> KRNYILGLAIGITSVGYGIIDYETRDVIDAGVRLFKEANVENNEGRRSKRGARRLKRRRRHRIQRVKKLLFDYNLLTDHSELSGINPYEARVKGLSQKLSEEEFSAALLHLAKRRGVHNVNEVEEDTGNELSTKEQISRNSKALEEKYVAELQLERLKKDGEVRGSINRFKTSDYVKEAKQLLKVQKAYHQLDQSFIDTYIDLLETRRTYYEGPGEGSPFGWKDIKEWYEMLMGHCTYFPEELRSVKYAYNADLYNALNDLNNLVITRDENEKLEYYEKFQIIENVFKQKKKPTLKQIAKEILVNEEDIKGYRVTSTGKPEFTNLKVYHDIKDITARKEIIENAELLDQIAKILTIYQSSEDIQEELTNLNSELTQEEIEQISNLKGYTGTHNLSLKAINLILDELWHTNDNQIAIFNRLKLVPKKVDLSQQKEIPTTLVDDFILSPVVKRSFIQSIKVINAIIKKYGLPNDIIIELAREKNSKDAQKMINEMQKRNRQTNERIEEIIRTTGKENAKYLIEKIKLHDMQEGKCLYSLEAIPLEDLLNNPFNYEVDHIIPRSVSFDNSFNNKVLVKQEEASKKGNRTPFQYLSSSDSKISYETFKKHILNLAKGKGRISKTKKEYLLEERDINRFSVQKDFINRNLVDTRYATRGLMNLLRSYFRVNNLDVKVKSINGGFTSFLRRKWKFKKERNKGYKHHAEDALIIANADFIFKEWKKLDKAKKVMENQMFEEKQAESMPEIETEQEYKEIFITPHQIKHIKDFKDYKYSHRVDKKPNRELINDTLYSTRKDDKGNTLIVNNLNGLYDKDNDKLKKLINKSPEKLLMYHHDPQTYQKLKLIMEQYGDEKNPLYKYYEETGNYLTKYSKKDNGPVIKKIKYYGNKLNAHLDITDDYPNSRNKVVKLSLKPYRFDVYLDNGVYKFVTVKNLDVIKKENYYEVNSKCYEEAKKLKKISNQAEFIASFYNNDLIKINGELYRVIGVNNDLLNRIEVNMIDITYREYLENMNDKRPPRIIKTIASKTQSIKKYSTDILGNLYEVKSKKHPQIIKKG

Staphylococcus aureus Cas9 (SaCas9) is a widely used genome editing tool. The CRISPR-Cas9 system has been emerging as a simple and powerful genome editing technology and is widely applied to the fields of gene therapy, drug screening, disease model construction, etc.. This system mainly consists of two components: Cas9 endonuclease and single-guide RNA (sgRNA). Additionally, its DNA editing process is roughly as follows: firstly, Cas9 binds to sgRNA to form a ribonucleoprotein (RNP) complex; next, the RNP searches for the protospacer-adjacent motif (PAM) on DNA to locate the target site; meanwhile, ~20 nt guide sequence of the sgRNA tries to pair with the DNA sequences upstream of the PAM; once they are in a form of base pairing, Cas9 endonuclease is activated and then precisely cleaves the target site.

To promote the stable binding of the protein to DNA, we mutated D10 and N580 of the wild-type SaCas9 (wtSaCas9) into alanine and obtained dead SaCas9 (dSaCas9). In this study, we report the first cryo-electron microscopy (cryo-EM) map of the SaCas9-sgRNA-DNA ternary complex. This map reveals that the HNH nuclease domain is tightly bound to the cleavage site of the target DNA strand and closely interacts with the WED and REC domains. Hence, most parts of the SaCas9-sgRNA-DNA complex are distributed in the high-resolution regions of the map, except for the HNH domain, L1/L2 linkers, and a small part of RuvC3 (aa 717–755). The components of the complex model are SaCas9 (aa 2-1053; D10A/N580A), 104 nt sgRNA, 40 nt target DNA strand, and 28 nt non-target DNA strand. In addition, the model shows that the cryo-EM density contacts of the HNH domain with the REC and WED domains are attributed to the hydrogen bonding between the domains: S581 of the HNH domain with E131 of the REC domain, and S595 and R586 of the HNH domain with K811 and D812 of the WED domain, respectively. The model shows that the non-target DNA strand fragment of the PAM upstream stably inserts into the positively charged groove formed by the HNH, L2, RuvC, and PI domains. Significantly, the full-length model also showed the hairpin structure of the stem-loop 2 in the sgRNA and revealed that the stem-loop 2 binds tightly to the positively charged groove formed by the PI and RuvC II domains. In addition, we observed that the double helix in the downstream of PAM is also embedded in the positively charged groove of the PI domain, and the phosphate backbone of dA15 in the target DNA strand binds to K1023 with a hydrogen bond. Site-directed mutagenesis and molecular dynamics (MD) simulations confirmed that the interactions of the HNH domain with the WED and REC domains are important for the DNA cleavage.>[3x]MVKNDYDLKFNPDKYISKEIKINGKKIKYRAYENIIYIKNPIDKDY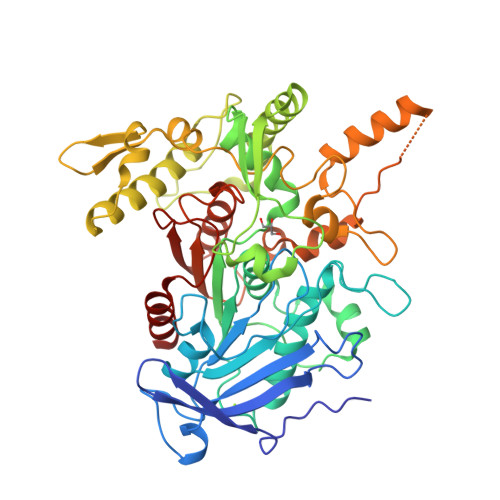QNMNIYIPEEYFNNLSIGSYNSNNAPIFFPNTVGGYMPGKADTVGLGRDGKANSLTYALSKGYVVAAPGARGRTLTDDKGNYIGKAPAAIVDLKAAVRYLYLNDEVMPGDANKIISNGTSAGGALSALLGASGNSQDYLPYLKEIGAAETRDDIFAVSAYCPITNLENADSAYEWMYNGVNSYSRMEFTRNTSAQEYNDRSLTRSTVQGNLTNDEINISNKLKTLFPIYLNSLKLTDDGGNLLTLDKSGNGSFKTYLSIIIRNSANRALREGKDISQFKKAFTIENNKVVAVNLDVYTHIGDRMKSPPAFDSLDASSGENNLFGDKKSDSKHFTKFSFDINNKAAIDYFRNGKFNDKNNKISIPKMADKNIIKMMNPMYYIDSNTSTKYWRIRHGAIDKDTSLAIPAILALKLKNSGKIVNFAAPWGQGHGGDYDLEELFNWIDNVVKK>MTTPTLIRRVSIEALDIPLHEPFGIAGGAQERAANLLVTVELADGTLGFGEAAPLPAFNGETQDGSRAAAVSLREAVVGSDARAWRAVARALREASGGGAGAARCAIETAILDALTKRAGMPLWAFFGGSGTALTTDITITTGSPERAEEAARRAAAMGFRALKVKVGGRLAASDPARIEAIHAAA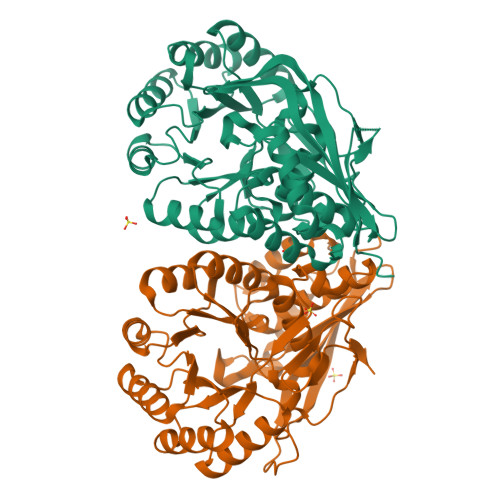PGASLILDGNGGLTAGEALALVAHARRLGADVALLEQPVPRDDWDGMKEVTRRAGVDVAADESAASAEDVLRVAAERAATVVNIKLMKGGIAEALDIAAVARAAGLGLMIGGMVESVLAMTASACFAAGLGGFSFVDLDTPLFLAENPFDGGFVQRGPALSLEGIRAGHGVTPQRRSPAAGAENLYFQSHHHHHHWSHPQFEK[2x]>[2x]MANRSIRDGDNPELLEERRM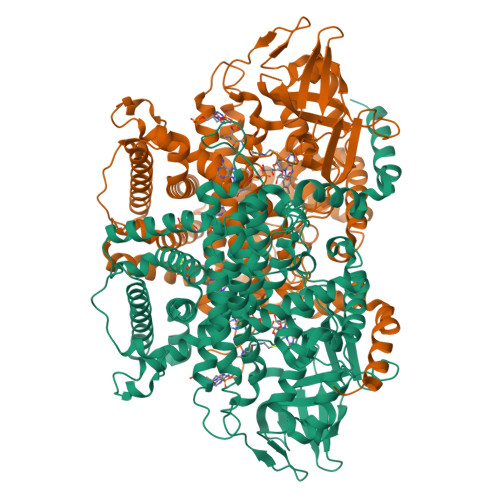ATFDTDKMAAVIYGSEEFARRRREITDAVSKIPELADIKPYPFLTREEKVTEGTRKISILTKYLNQLIDRDNEEESLHLHREVIGYEGHPFALHDALFIPTLQSQASDEQQEKWLERARRREIIGCYAQTELGHGSNLRNLETTAVYDIASQEFVLHTPTTTALKWWPGALGKSCNYALVVAELIIKRNNYGPHFFMVQLRDEKTHIPLKGVTVGDIGPKMNFNAADNGYLGLNNLRVPRTNLLMRHCKVEADGTYVKPPHAKIGYSGMVKIRSQMAMEQGLFLAHALTIAARYSAVRRQGHLDDKQVEVKVLDYQTQQHRLFPSLARAYAFIFTGFETIHLYSQLLKDVDMGNTSGMADLHALTSGLKSVVAHETGEGIEQARMACGGHGYSMASYISVVYGIAIGGCTYAGENMVMLLQLARYLVKSVELIKAGKAKKLGPVASYLADKSDETDLTSLNGYVKMFENMARRQAWKATEKFLKLMESGESREVAWNKSAVELTRASRLHTRLFIIEAFMRRVSRIEDIPVKEVLTDLLHLHVNYELLDVATYALEFMSFTQLDYVRDQLYLYLEKIRPNAVSLVDSFQISDMQLRSVLGRRDGHVYENLFKWAKSSPLNNADVLPSVEKYLKPMMEKAKLAAAHHHHHHHHHH>DDVVTFKAQEQLQRASEQAHNSPVLRALLAESLRLFEQVAGSLTPANLTTAVEQYISLKYYAGAIQLCLTVAQQKDRGNTALSWVNDGKPANDSRKKAFDERKICYNLIHQVLDKLESDFAGEPELVDGRPTLAATKRMEAYNVVNDSSDEVFHFDLYEWYIEKGWTDRILSIDSPHVITYLQRLAETDFRHAELLCRFYTTRSRFFEAAQVQTNLAKSDLNISLKDRIILLSRAKGNASVNTIGISRQQQQQLNHEASELLEIAHIQDDLLERLVADPRIPEERKAEIEEFLDGPIRTLTDLFNDYADQANYYDLCLLIFHAADFHNPRTILDTWNNLINQSHFEAEQRREYWEIVQAGGDLPAGVIAPIAEPPLPYVYVSQQIQLIAHRTSLDSLIFPVNSLLPVVCAYAINNGQDASIGADPCWPIQLFLNLGVPHALVVQVLENVLDTQEAPFTGRRRKLVVQWIAMAVDMWVREVERRGAMAAAAASGASGSEAVMGSWVSELLGRADQVLTQIAGTGAGGAASDAEEIASLRRTVKGLK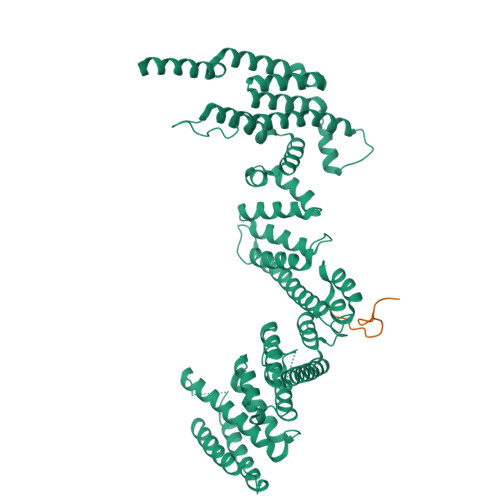RSVD[4x];>SHKKLVINKDMRTDLFSPPNKD[4x]> MAIYADNSYSIGNTPLVRLKHFGHNGNVVVKIEGRNPSYSVKCRIGANMVWQAEKDGTLTKGKEIVEPTSGNTGIALAYVAAARGYKITLTMPETMSIERKRLLCGLGVNLVLTEGAKGMKGAIAKAEEIVASDPSRYVMLKQFENPANPQIHRETTGPEIWKDTDGKVDVVVAGVGTGGSITGISRAIKLDFGKQITSVA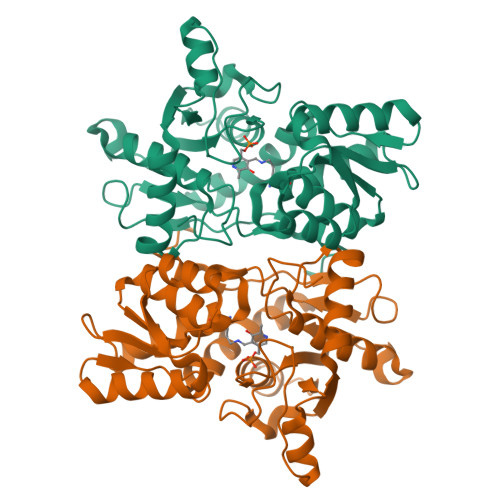VEPVESPVISQTLAGEEVKPGPHKIQGIGAGFIPKNLDLSIIDRVETVDSDTALATARRLMAEEGILAGISSGAAVAAADRLAKLPEFADKLIVVILPSSSERYLSTALFEGIEG>[2x]MAEIGTGFPFDPHYVEVLGERMHYVDVGPRDGTPVLFLHGNPTSSYVWRNIIPHVAPTHRCIAPDLIGMGKSDKPDLGYFFDDHVRFMDAFIEALGLEEVVLVIHDWGSALGFHWAKRNPERVKGIAFMEFIRPIPTWDEWPEFARETFQAFRTTDVGRKLIIDQNVFIEGTLPMGVVRPLTEVEMDHYREPFLNPVDREPLWRFPNELPIAGEPANIVALVEEYMDWLHQSPVPKLLFWGTPGVLIPPAEAARLAKSLPNCKAVDIGPGLNLLQEDNPDLIGSEIARWLSTLEISGHHHHHH

Here we present a GSH-sensing platform for live-cell imaging, termed targetable ratiometric quantitative GSH (TRaQ-G). We hypothesized that a SiR dye in a spirocyclic form would be non-reactive against GSH, but it could isomerize to its zwitterionic form upon binding to the self-labelling protein HaloTag (HT), switching both its fluorescence and reactivity against GSH from an ‘off’ to an ‘on’ state. In conclusion, we have designed, synthesized and validated a new ratiometric GSH sensor, TRaQ-G, which only becomes reactive in the organelle of interest. This sensor is based on binding of a spirocyclic SiR ligand to HT, which induces isomerization to the GSH-sensitive and fluorescent zwitterionic form. We conducted X-ray diffraction experiments and MD simulations for structural elucidation of the different TRaQ-G adducts to gain mechanistic insight into the varying GSH sensitivities of the molecules.

Our first goal was to demonstrate that a known SiR-based GSH sensor, QG3.013, retained its reactivity towards GSH when bound to HT. We therefore substituted the reference fluorophore of QG3.0 with a chloroalkane linker, a substrate that reacts with HT. The SiR unit was synthesized according to the reported procedure, and the linker was attached via amide coupling to give the Me–TRaQ-G ligand. Using this molecule, we prepared and purified the HT adduct, Me–TRaQ-G. The reactivity of Me–TRaQ-G against GSH was nearly identical to that of QG3.0, suggesting that one face of the xanthene π-system of Me–TRaQ-G must be exposed to the solvent, thus allowing for GSH nucleophilic attack. This hypothesis was confirmed by X-ray diffraction studies of the adduct, which revealed that the methyl group of the Me–TRaQ-G ligand fits into a shallow hydrophobic pocket created by residues F152, V167 and T172 of HT, exposing the opposite face of the xanthene core to the solvent. Although Me–TRaQ-G is sensitive towards GSH, we envisioned that it would perform poorly in live cells given its constant fluorescence and reactivity towards GSH. This suspicion was confirmed by imaging cells expressing HT in the nucleus, which revealed unacceptable levels of off-target signals.>MDTAGDTKTTDDGGVVNITYMHRLPDSEGMTLVNDIVAKWNKQHPDIQVKATKFDGKASDMIKKLETDVKSGEAPDLAQVGYAELPEVFTKGLLQDVTQYAEQYKNDFASGPYSLVQVGGKAYGLPQDTGPLVYFYNKAEFEKLGITEIPQTADEFIAAAKTAAAAGKYIMSYQPDEAGNMISGLAGASGGWYKVKGDSWVVNTETDGSKATADFYQQLLDAKAATTNPRWDPSFDASIKDGSLIGTVAAAWEAPLFMTSSGGTGSGEWQVAQLGDWFGNAGKTGPDGGSAVAVLKNSKHPKEAMEFLDWFNTQVPDLVSQGLVPAATTEDAETPSEWSTFFGGQDIMKEFKTAN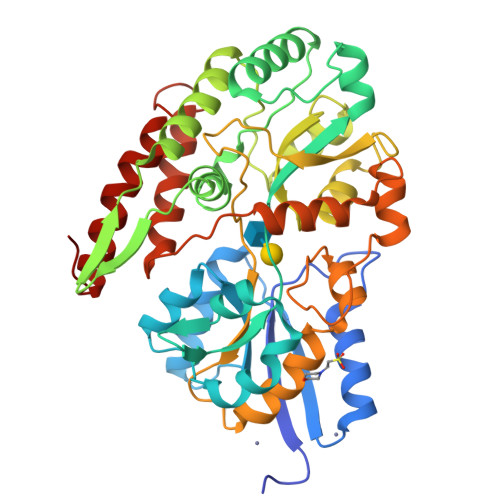NNMGDFTYMPGFSAVAAKMNETAAKATDGSGKVADIFSDAQTTSVDTLKNFGLSVSE[2x]> MSKLELLPAVDVRDGQAVRLVHGESGTETSYGSPLEAALAWQRSGAEWLHLVDLDAAFGTGDNRALIAEVAQAMDIKVELSGGIRDDDTLAAALATGCTRVNLGTAALETPEWVAKVIAEHGDKIAVGLDVRGTTLRGNGWTRDGGDLYETLDRLNKEGCARYVVTDIAKDGTLQGPNLELLKNVCAATDRPVVASGGVS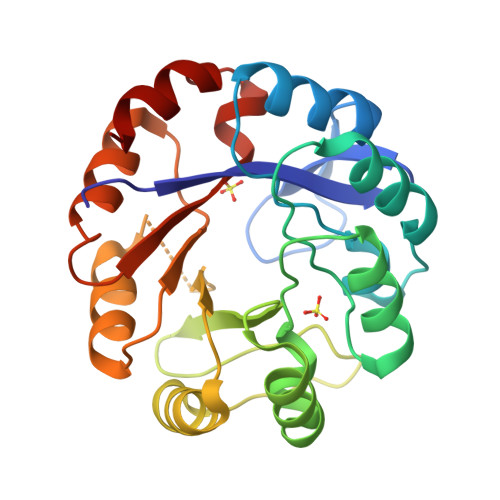SLDDLRAIAGLVPAGVEGAIVGKALYAKAFTLEEALEATS NoVs are encapsulated by a protein capsid that is assembled by a single major structural protein, the capsid protein VP1. VP1 is divided into the N-terminal shell (S) and the C-terminal protruding (P) domain, forming the interior shell and the multiple protrusions of the capsid, respectively. HuNoVs interact with histo-blood group antigens (HBGAs) in a strain-specific manner. In this study, through X-ray crystallography of the P domain of a GII.21 huNoV (OIF) we identified a unique lineage in GII consisting of GII.13 and GII.21 genotypes that recognize HBGAs through a binding interface distinct from the GII conventional binding interface.

The crystal of the native P domain protein belongs to the P21 space group, with two monomers forming a dimer in an asymmetric unit. The final refined structure of native P domain includes residues 223 to 527, with the exception of a loop region comprising residues 340~342 due to the lack of recognizable electron density. The two monomers of the OIF P dimer are related by a non-crystallographic two-fold axis, which forms the biologically active protrusion of the NoV capsid. The P dimer has a dimension of 55 Å×64 Å×70 Å with an extensively buried interface of 3,500 Å2 between two protomers, including hydrophobic and hydrophilic interacting residues from both P1 and P2 subdomains. The P-loop of the OIF P dimer exhibits a unique conformation, taking a ~90° flip, which results in its extruding out of the flat surface and approaching the opposite protomer. As a result, the majority of the S-loop is covered in the OIF virus. Such structural rearrangements destroy the structural integrity of the conventional GII HBGA binding interfaces that are formed mainly by P- and S-loops. On the other hand, the B- and the T-loops also exhibit unique conformations, approaching to each other in closer proximity with the N-loop. This special structural feature allows the formation of new HBGA binding interface (see below), formed by the B-, T- and N-loops, a scenario that is absent in all other known GII huNoV structures. Analysis of the native OIF P domain structure revealed that a glycerol molecule occupies the HBGA binding pocket, which was clearly visible from the 2Fo-Fc omit map. The glycerol molecule is held firmly inside the HBGA binding pocket by eight direct hydrogen bonds between the hydroxyl groups of the glycerol and the side chains of N392, N394 and T395 from the T-loop, T356 and the main chain of S357 from the N-loop. Interestingly, the glycerol molecule resembles partial structures (C2, C3, and C4 with their hydroxyl groups) of the β-Gal that contributes the vast majority of the interactions with the binding pocket (Compare Fig 5F with Fig 7C), thus explaining the observed interactions.

>GPLGSPEFSKTKPFTLPILTIGELTNSRFPAPIDQLYTSPNADVVVQPQNGRCSLDGELQGTTQLLTTAICSYRGMTSNPTRDYWDGHLLHLVHPNGATYDPTEDVPAPFGTQDFRGILYGVLTQNPRASGDEAANSQGVYISSTSEKFTPKLGTIGLHQVQGNIASNQQSKFTPVGIAVNGNTPFRQWELPNYSGALTLNTNLAPAVGPNFPGEQILFFRSNVPSVQGGQPIEIDCLIPQEWVSHFYQESAPSQSDVALVRYVNPDTGRTIFEAKLHRQGFITIAATGSNPVVVPPNGYFRFDSWVNQFYALAPM[2x]> ETGTPMMPPVGVQASILSHDTIRITWADNSLPKHQKITDSRYYTVRWKTNIPANTKYKNANATTLSYLVTGLKPNTLYEFSVMVTKGRRSSTWSMTAHGATFELVPTSPPKDVTVVSKEGKPRTIIVNWQPPSEANGKITGYIIYYSTDVNAEIHDWVIEPVVGNRLTHQIQELTLDTPYYFKIQARNSKGMGPMSEAVQFRTPKADSSDKMPNDQALGSAGKGSRLPDLGSDY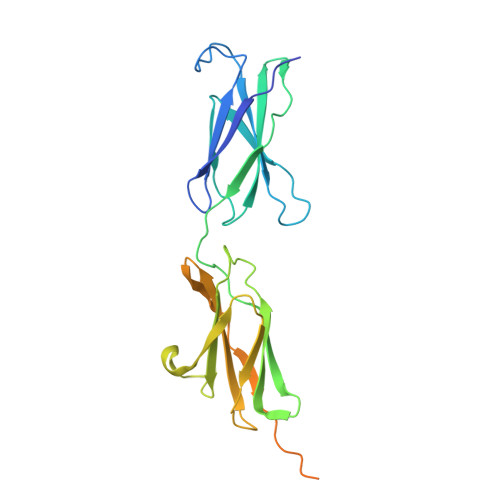KPPMSGSNSPHGSPTSPLDSNGTKHHHHHH> GGMGQTLLDALNVRVVGSGERVLVLAHGFGTDQSAWNRILPFFLRDYRVVLYDLVCAGSVNPDFFDFRRYTTLDPYVDDLLHILDALGIDCCAYVGHSVSAMIGILASIRRPELFSKLILIGASPRFLNDEDYHGGFEQGEIEKVFSAMEANYEAWVNGFAPLAVGADVPAAVREFSRTLFNMRPDITLFV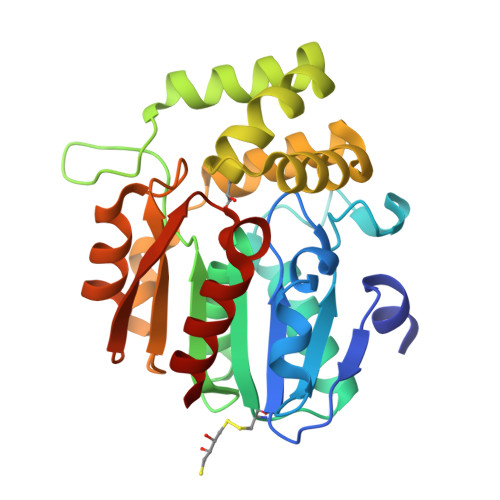SRTVFNSDMRGVLGLVKVPCHIFQTARDHSVPASVATYLKNHLGGKNTVHWLNIEGHLPHLSAPTLLAQELRRALSHR>[4x]GEAQPASGRFDQVGGAFGWKPHKLDPKECAQVAYDGYWYKGF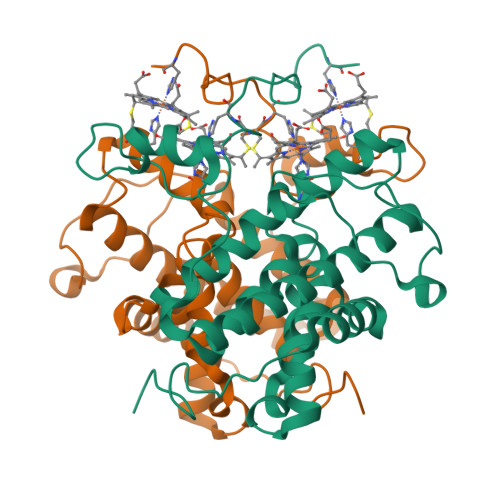GCGFGAFYSIVGLMGEKYGAPYNQFPFAMLEANKGGISDWGTICGALYGAAATFSLFWGRKEVHPMVNELFRWYEVTKLPIFNPGDAAQGVKGDLPMSASDSVLCHISVSKWCYENKIEATSKQRSERCGRLTADAAFKAAEIINTKIDQGKDFKSTFPMQASVSSCGECHMTKGNDANWAKGIMDCTPCHSGTAATQNKFVNHP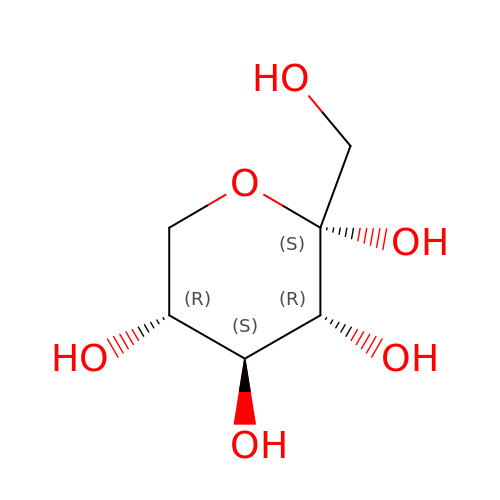alpha-D-Sorbopyranose | C6 H12 O6 | LKDRXBCSQODPBY-MOJAZDJTSA-N> ANQEIFDKLRDAIVNQNVAGTP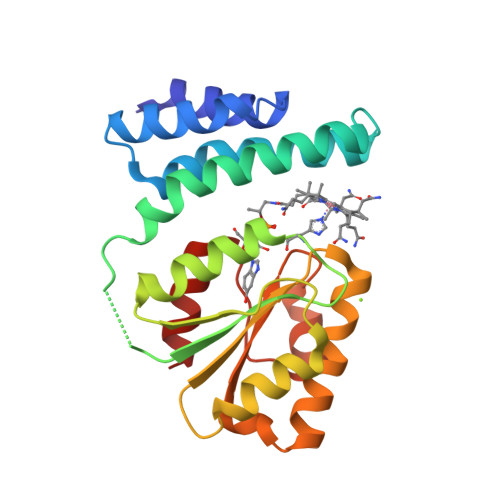ELCKEALAAGVPALDIITKGLSVGMKIVGDKFEAAEIFLPQIMMSGKAMSNAMEVLTPELEKNKKEGEEAGLAITFVAEGDIHDIGHRLVTTMLGANGFQIVDLGVDVLNENVVEEAAKHKGEKVLLVGSALMTTSMLGQKDLMDRLNEEKLRDSVKCMFGGAPVSDKWIEEIGADATAENAAEAAKVALEVM4-[3-amino-6-(3,4,5-trimethoxyphenyl)pyrazin-2-yl]-2-ethoxybenzoic acid | C22 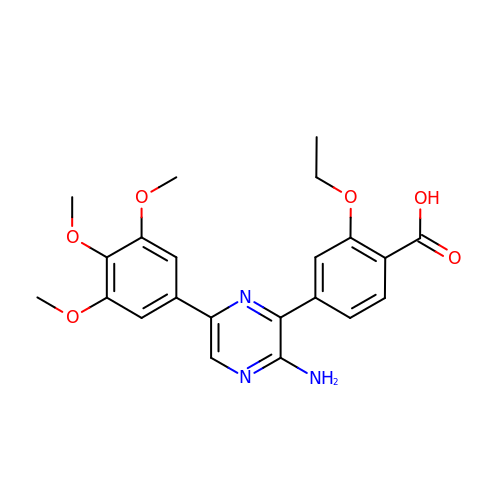H23 N3 O6 | MVWFAKKKMGICFP-UHFFFAOYSA-N Apical localization of the Crumbs (Crb) transmembrane protein requires a PDZ-mediated interaction with Pals1 (protein-associated with Lin7, Stardust, MPP5), a member of the p55 family of membrane-associated guanylate kinases (MAGUKs). Pals1 belongs to the MPP family of proteins (membrane protein, palmitoylated), also known as the p55 subfamily of membrane-associated guanylate kinases (MAGUKs). Pals1 acts as a scaffold protein, recruiting other proteins to the apical domain of the cells: the L27 domains of Pals1 bind to Patj and Lin7, while the amino-terminal regions of Pals1 can interact with the PDZ domain of Par6, linking the Crb and Par complexes.

In order to investigate the conformational changes that occur in Pals1PDZ upon binding Crb17 peptide, a ligand-free form of Pals1PDZ was crystallized and its structure was determined at 1.8 Å resolution. This crystal form has a single copy of Pals1PDZ in the asymmetric unit. The structure of ligand-free Pals1PDZ reveals a sterically blocked peptide-binding groove, as confirmed by fluorescence polarization in vitro. Firstly, the carboxylate-binding β1–β2 loop (residues 260–268) adopts a more open configuration pivoting at Glu260 and Leu267, resulting in a Cα shift of over 6.2 Å away from the C-terminal end of helix α2. This exposes the side chain of Pals1 Lys261 and ensures that this part of the PBM-binding groove is solvent-accessible. The Leu321 side chain adopts a favoured rotamer in the absence of a partner peptide. The Phe318 side-chain rotamer adopted in the apo Pals1PDZ results in a steric block to the central part of the PDZ peptide-binding groove. We therefore considered whether Phe318 could act as a potential gating mechanism restricting access of ligand to the PDZ peptide groove. We note that the ligand-free Pals1 PDZ domain closely resembles that of Par6, which is known to bind both internal and C-terminal peptide ligands. Examination of the open carboxylate-binding loop of ligand-free Pals1 PDZ domain with Par6 bound to an internal peptide ligand suggests that Pals1 could also bind internal ligands.

> GPLGSGETVKIVRIEKARDIPLGATVRNEMDSVIISRIVKGGAAEKSGLLHEGDEVLEINGIEIRGKDVNEVFDLLSDMHGTLTFVLIPS>MSHLENCLGVQKIAPEQIRQLFAQTSEYHFSIPAKTEEKSNLNVFFGEGRRD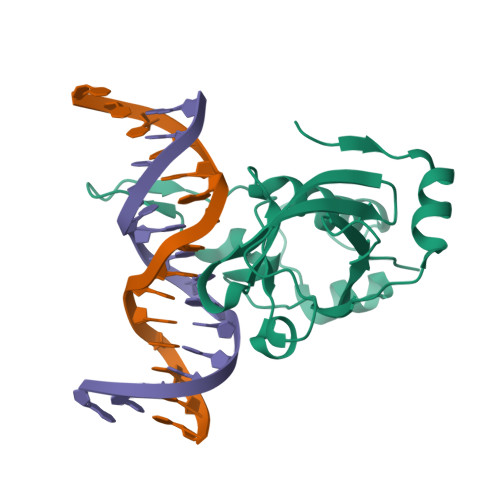KRGFVKPRPWYEVELIVSKDITSQEGYPVLKSFTVITDDGWQFQCKTSGDYSKNFRSENDLKTLGKWIKGRLESHGCLQNNEKITHETLREYGNDHFELRSTDNPDVWLLSFKGKNSGGHHHHHHG[2x]> MSLSNGELAILVFGYPETMANQVIAYFQEFGTILEDFEVLRKPQAMTVGLQDRQFVPIFSGNSWTKITYDNPASAVDALLENGA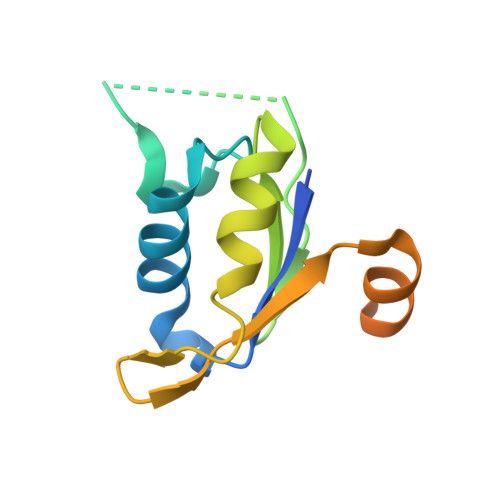VFNGVLLGVIPYTKDAVERLQKRKLTSSEDIGSGITTAAAEGHHHHHH>[2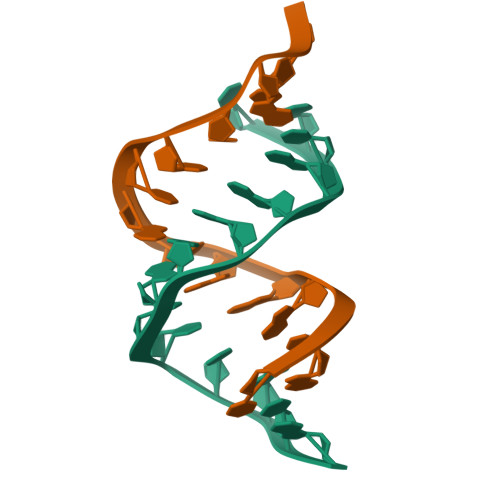x]CGCGGGTACCCGCG>[2x]DPFTMMILKIGGSVITDKSAYRTAR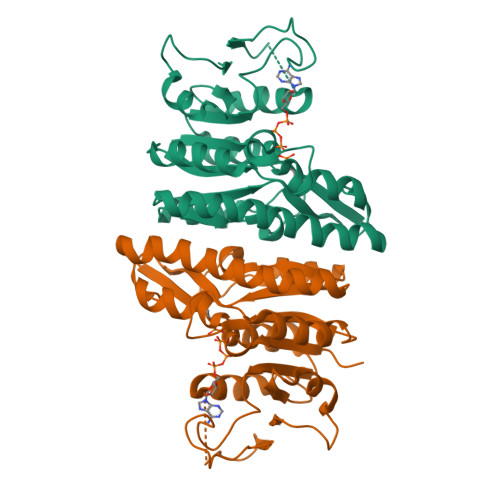TYAIRSIVKVLSGIEDLVCVVHGGGSFGHIKAMEFGLPGPKNPRSSIGYSIVHRDMENLDLMVIDAMIEMGMRPISVPISALRYDGRFDYTPLIRYIDAGFVPVSYGDVYIKDEHSYGIYSGDDIMADMAELLKPDVAVFLTDVDGIYSKDPKRNPDAVLLRDIDTNITFDRVQNDVTGGIGKKFESMVKMKSSVKNGVYLINGNHPERIGDIGKESFIGTVIR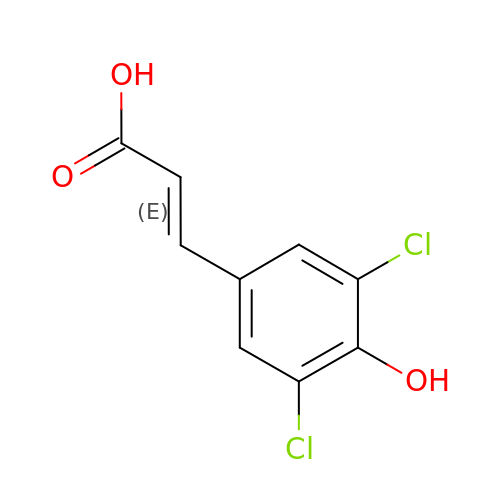(2E)-3-(3,5-dichloro-4-hydroxyphenyl)prop-2-enoic acid | C9 H6 Cl2 O3 | YCWRKUFHHMQSOU-OWOJBTEDSA-N> MASPAAGDVLIVGSGLVGRSWAMLFASGGFRVKLYDIEPRQITGALENIRKEMKSLQQSGSLKGSLSAEEQLSLISSCTN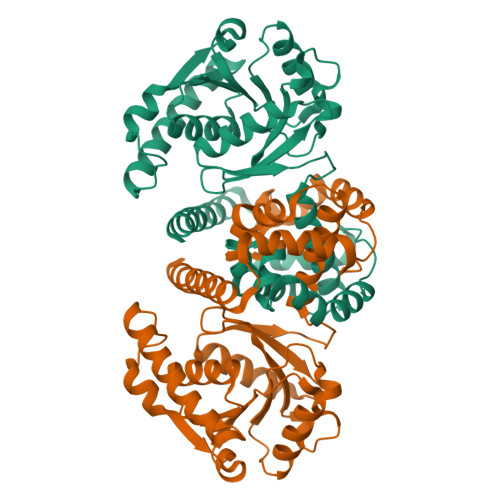LAEAVEGVVHIQECVPENLDLKRKIFAQLDSIVDDRVVLSSSSSCLLPSKLFTGLAHVKQCIVAHPVNPPYYIPLVELVPHPETSPATVDRTHALMRKIGQSPVRVLKEIDGFVLNRLQYAIISEAWRLVEEGIVSPSDLDLVMSDGLGMRYAFIGPLETMHLNAEGMLSYCDRYSEGMKRVLKSFGSIPEFSGATVEKVNQAMCKKVPADPEHLAARREWRDECLKRLAKLKRQMQPQ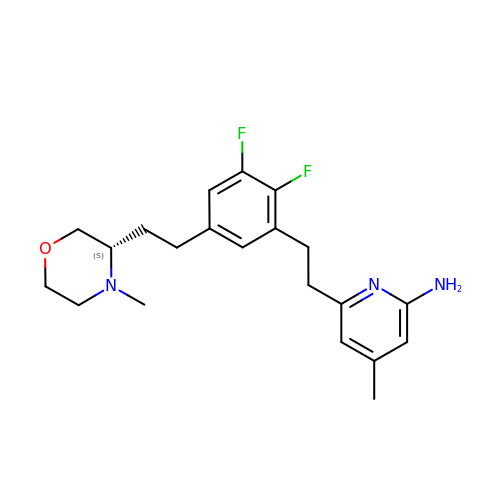6-[2-(2,3-difluoro-5-{2-[(3S)-4-methylmorpholin-3-yl]ethyl}phenyl)ethyl]-4-methylpyridin-2-amine | C21 H27 F2 N3 O | WLROZYRNCCIRPN-SFHVURJKSA-N>MRRNIFCLACLWIVQACLSLDRADILYNIRQTSRPDVIPTQRDRPVAVSVSLKFINILEVNEITNEVDVVFWQQTTWSDRTLAWNSSHSPDQVSVPISSLWVPDLAAYNAISKPEVLTPQLARVVSDGEVLYMPSIRQRFSCDVSGVDTESGATCRIKIGSWTHHSREISVDPTTENSDDSEYFSQYSRFEIL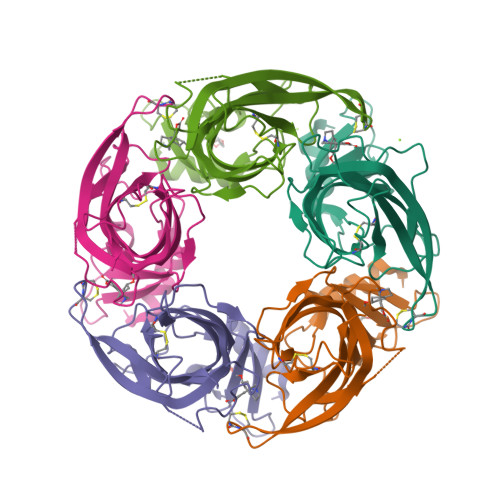DVTQKKNSVTYSCCPEAYEDVEVSLNFRKKGRSEIL[10x]> MAEYKDNLLGEANSFLEVLEQVSHLAPLDKPVLIIGERGTGKELIASRLHYLSSRWQGPFISLNCAALNENLLDSELFGHEAGAFTGAQKRHPGRFERADGGTLFLDELATAPMMVQEKLLRVIEYGELERVGGSQPLQVNVRLVCA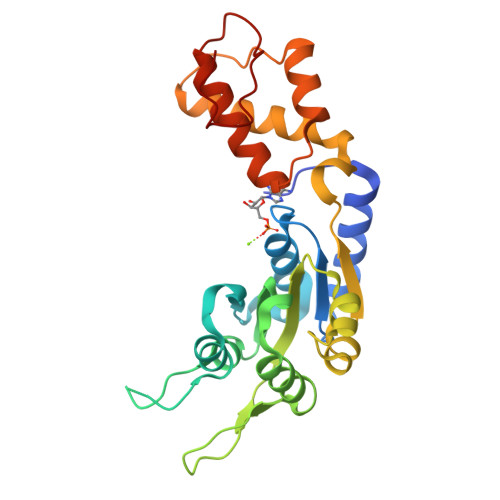TNADLPAMVNEGTFRADLLDRLAFDVVQLPPLRERESDIMLMAEYFAIQMCREIKLPLFPGFTERARETLLNYRWPGNIRELKNVVERSVYRHGTSDYPLDDIIIDPFKRRP>[2x]RGSHHHHHHGSMGDNIVLYYFDARGKAELIRLIFAYLGIEYTDKRFGVNGDAFVEFKNFKKEKDTPFEQVPIL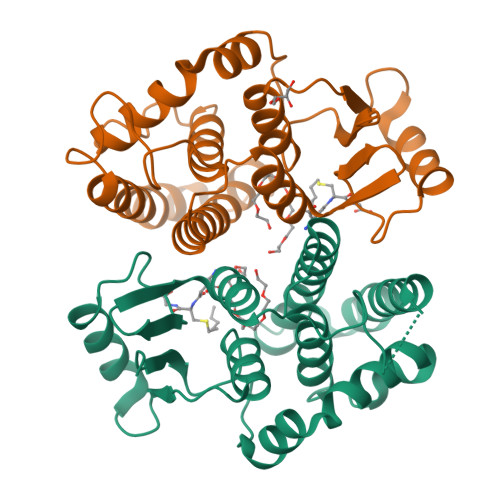QIGDLILAQSQAIVRYLSKKYNICGESELNEFYADMIFCGVQDIHYKFNNTNLFKQNETTFLNEDLPKWSGYFEKLLKKNHTNNNNDKYYFVGNNLTYADLAVFNLYDDIETKYPSSLKNFPLLKAHNEFISNLPNIKNYITNRKESVY> SPVEWTVMDVVEYFTEAGFPEQATAFQEQEIDGKSLL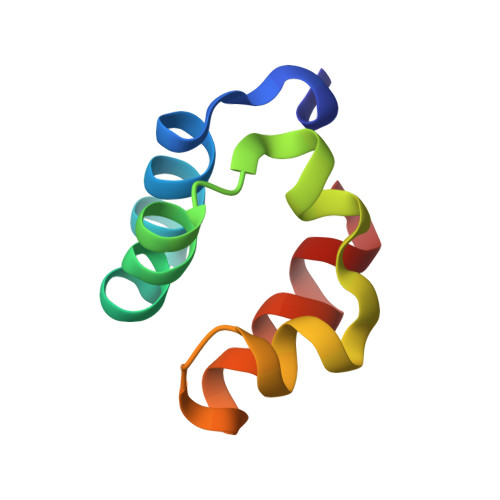RMQRTDVLTGLSIRLGPALKIYEHHIKVL>GLASLADFPIGVAVAASGGNADIFTSSARQNIVRAEFNQITAENIMKMSYMYSGSNFSFTNSDRLVSWAAQNGQTVHGHALVWHPSYQLPNWASDSNANFRQDFARHIDTVAAHFAGQVKSWDVVNEALFDSADDPDGRGSANGYRQSVFYRQFGGPEYIDEAFRRARAADPTAELYYNDFNTEENGAKTTALVNLVQRLLNNGVPIDGVGFQMHVMNDYPSIANIRQAMQKIVALSPTLKIKITCLDVRLNNPYDGNSSNDYTNRNDCAVSCAGLDRQKARYKEIVQAYLEVVPPGRRGGITVWGIADPDSWLYTHQNLPD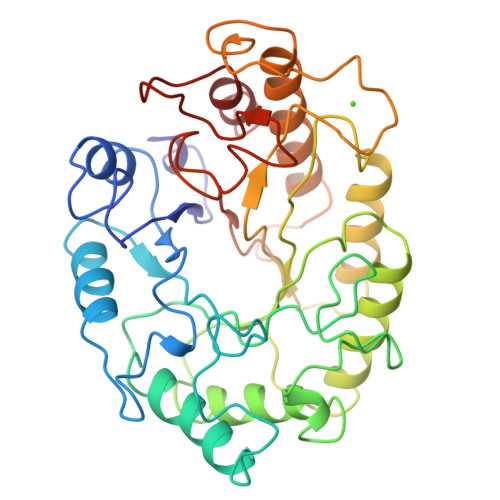WPLLFNDNLQPKPAYQGVVEALSGR[2x]>[3x]MGHHHHHHSHMAVADLALIPDVDIDSDGVFKYVLIRVHSAPRSGAPAAESKEIVRGYKWAEYHADIYDKVSGDMQKQGCDCECLGGGRISHQSQDKKIHVYGYSMAYG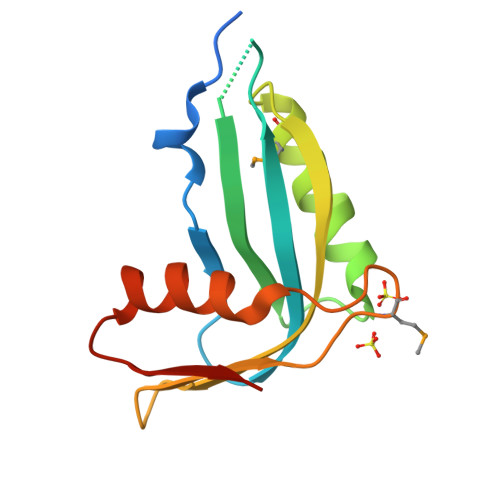PAQHAISTEKIKAKYPDYEVTWANDGY>VDFHGYARSGIGWTGSGGEQQCFQTTGAQSKYRLGNECETYAELKLGQEVWKEGDKSFYFDTNVAYSVAQQNDWEATDPAFREANVQGKNLIEWLPGSTIWAGKRFYQRHDVHMIDFYYWDISGPGAGLENIDVGFGKLSLAATRSSEAGGSSSFASNNIYDYTNETANDVFDVRLAQMEINPGGTLELGVDYGRANLRDNYRLVDGASKDGWLFTAEHTQSVLKGFNKFVVQYATDSMTSQGKGLSQGSGVAFDNEKFAYNINNNGHMLRILDHGAISMGDNWDMMYVGMYQDINWDNDNGTKWWTVGIRPMYKWTPIMSTVMEIGYDNVESQRTGDKNNQYKITLAQQWQAGDSIWSRPAIRVFATYAKWDEKWGYDYTGNADNNANFGKAVPADFNGGSFGRGDSDEWTFGAQMEIWW[3x]

Here, we tested a new tool to drive density fitting with molecular dynamics simulations, in the context of a new structure of the membrane protein maltoporin. Specifically, we collected and processed cryo-EM data for the E. coli membrane protein maltoporin, and we used a previously reported x-ray structure as a starting model to refine against the cryo-EM density in various environments. We present a protocol for using density-guided molecular dynamics simulations to automatically refine atomistic models into membrane protein cryo-EM maps. Membrane proteins are particularly important targets in pharmacology and bioengineering but present distinctive challenges to data quality and modeling.

In this work, we set out to determine the applicability of GROMACS density-guided simulations to automatically refine a membrane protein system. Using adaptive force density-guided simulations as implemented in the GROMACS molecular dynamics package, we show how automated model refinement of a membrane protein is achieved without the need to manually tune the fitting force ad hoc. The proposed protocol was used to refine models into a new cryo-EM density of the membrane protein maltoporin, either in a lipid bilayer or detergent micelle, and we found that results do not substantially differ from fitting in solution. Fitted structures satisfied classical model-quality metrics and improved the quality and the model-to-map correlation of the x-ray starting structure. Fitting performed well in detergent, lipids, or solution, offering simpler options for fully automated simulation protocols. We also present selection criteria to choose the best-fit model that balances stereochemistry and goodness of fit. Additionally, the density-guided fitting in combination with generalized orientation-dependent all-atom potential was used to correct the pixel-size estimation of the experimental cryo-EM density map. In addition to identifying a robust parameter set and model-quality metrics for refinement of membrane proteins, we report an improved estimation of the pixel size of cryo-EM data based on goodness of fit and stereochemistry of simulated models.>MEFGSFLVSLGTSFVIFVILMLLFTWLSRKSGNAPIYYPNRILKGLEPWEGTSLTRNPFAWMREALTSSEQDVVNLSGVDTAVHFVFLSTVLGIFACSSLLLLPTLLPLAATDNNIKNTKNATDTTSKGTFSQLDNLSMANITKKSSRLWAFLGAVYWISLVTYFFLWKAYKHVSSLRAQALMSADVKPEQFAILVRDMPAPPDGQTQKEFIDSYFREIYPETFYRSLVATENSKVNKIWEKLEGYKKKLARAEAILAATNNRPTNKTGFCGLVGKQVDSIEYYTELINESVAKLETEQKAVLAEKQQTAAVVFFTTRVAAASAAQSLHCQMVDKWTVTEAPEPRQLLWQNLNIKLFSRIIRQYFINFFVAVTILFYMIPIAFVSAITTLKNLQRIIPFIKPVVEITAIRTVLESFLPQIALIVFLAMLPKLLLFLSKAEGIPSQSHAIRAASSKYFIFSVFNVFIGVTLAGTLFNTVKDIAKNPKLDMIINLLATSLPKSATFFLTYVALKFFIGYGLELSRIIPLIIFHLKKKYLCKTEAEVKEAWYPGDLSYATRVPGDMLILTITFCYSVIAPLILIFGITYFGLGWLVLRNQALKVYVPSYESYGRMWPHIHQRILAALFLFQVVMFGYLGAKTFFYTALVIPLIITSLIFGYVCRQKFYGGFEHTALEVAC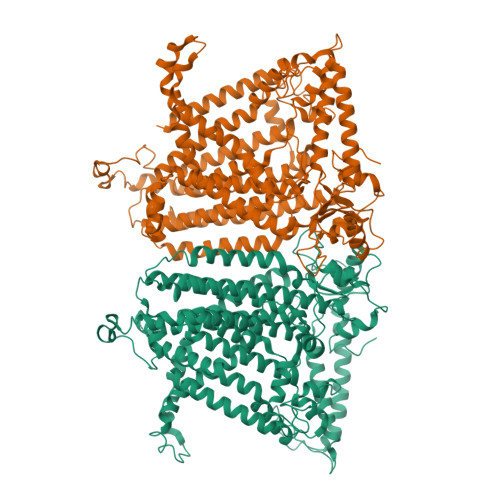RELKQSPDLEEIFRAYIPHSLSSHKPEEHEFKGAMSRYQDFNAIAGVSNSLEV[2x]> PSSTMGQVGRQLAIIGDDINR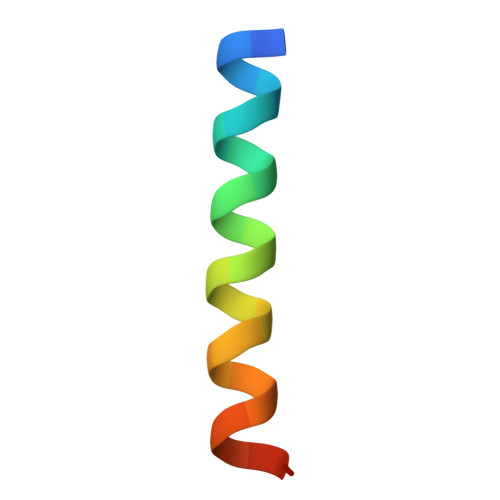RYDSE>GPMMATKGRLLTTPTRLLKLILPIPFHPEQEYINSDETKTNKPKEDAVEPLALLVHPQQPLSYLERLIQAEIPPLLVKDREKLPEIIFRAEADYTGGNGDTHWVRWSGSTEIGDFIRDAARGREFSVTIEGHAEELRVAVPSFKDRTYYMRMRLRRMSQEIDQ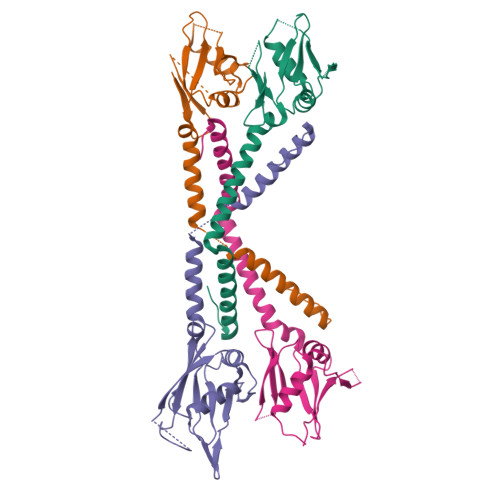MATVKREAKWDQLVHDANGLRREIKFAATEYGVEWDEMKDLGGEEVK[8x]>[2x]GAMGDILIVWAKDVDEMLKQVEILRRLGAKQIAVESSDWRILQEALKKGGDILIVNGGGMTITFRGDDLEALLKAAIEMIKQALKFGATITLSLDGNDLNINI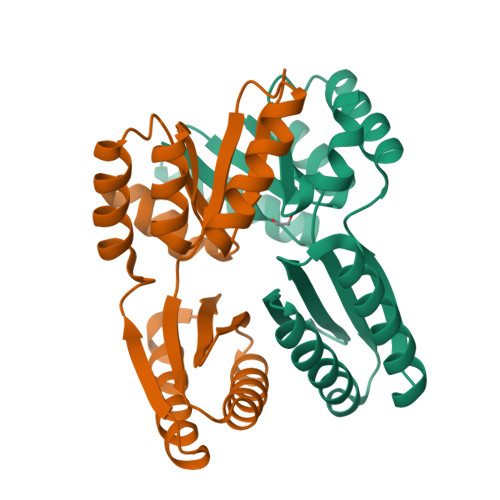TGVPEQVRKELAKEAERLAKEFGITVTRTGGGDVDEMLKQVEILRRLGAKQIAVESDDWRILQEALKKG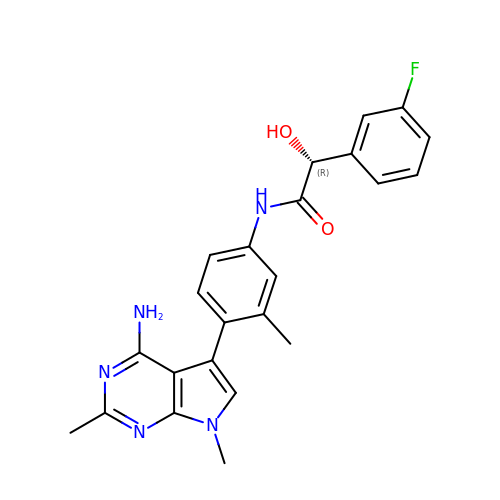(2R)-N-[(4M)-4-(4-amino-2,7-dimethyl-7H-pyrrolo[2,3-d]pyrimidin-5-yl)-3-methylphenyl]-2-(3-fluorophenyl)-2-hydroxyacetamide | C23 H22 F N5 O2 | NZUZHCPIKAILKT-HXUWFJFHSA-N>ASDASPIAYVNLPQAFVFNVTGDSRDRLVQIKAQLMVRGAENEELARYHSPLIESSLLSTFASAT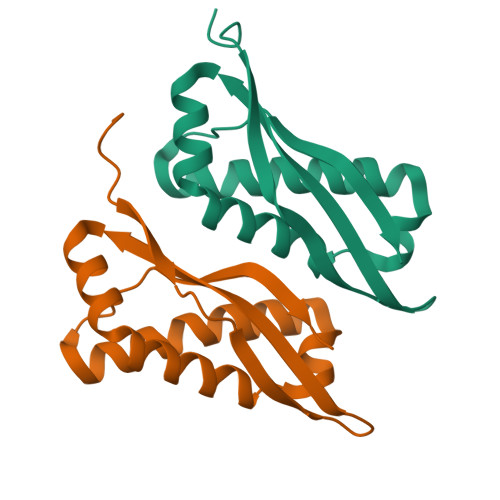VDQLRSPTGRVELRDRASEDIKAALNAAVGKPVIEKVLFTDFVIQ[2x]> GLYFPQRLYTENIYVGQQQGSPLLQVISMREFPTERPYFFLCSHRDAFTSWFHIDEASGVLYLNKTLEWSDFSSLRSGSVRSPKDLTLKVGVSSTPPMKVMCTILPTVEVKLSFINDTAPSCGQVELSTLCFPEKISNPHITENREPGALRQLRRFTHMSICPNYTISYGVVAGSSVPFAVDDSTSELVVTAQVDREEKEVYHLD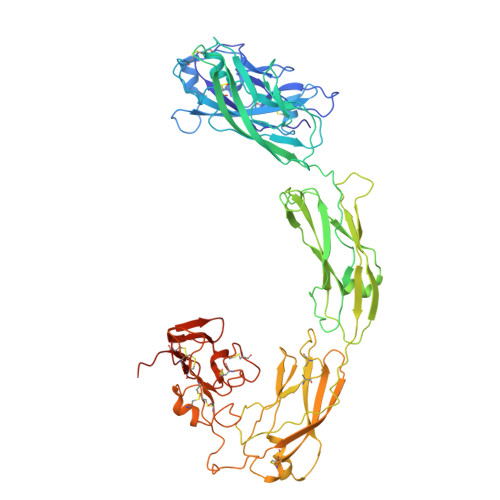IVCMVRTERNLEEVFRSLHVNIYDEDDNSPYVNGTDTEDVLVEFDRSEGTVFGTLFVYDRDTTPVYPTNQVQNKLVGTLMTNDSWIKNNFAIEHKFREEKAIFGNVRGTVHEYKLKLSQNLSVTEQRSFLLGYLVNDTTFPGPEGTVLLHFNVTVLPVPIRFSNVTYSFTVSQKATTYSQIGKVCVENCQKFKGIDVTYQLEIVDRNITAEAQSCYWAVSLAQNPNDNTGVLYVNDTKVLRRPECQELEYVVIAQEQQNKLQAKTQLTVSFQGEADSLRTDEPRFPACAEKRQRGDCEATRGLGAPTGRCQWRQGRDKGISKRYSTCSPNLGTCPDGYCDAIESKNISICPQDCSSEAIIGGYERDLYGIKAGHGTCYCFEGKCFCERDEPEDDICNDMCGSEFENLYFQ> SAGNDSLPFENIQGDILVGMKKDKEKFVFFHINNATAFKSVLKTYAPANITSVATIIGPVANQPLAFVNLAFSHAGFGALNVTDDLQDTAFSDGQFKDSPNLGDDTSTWEEAFKGTNVDGVFLIGSNDESITAQYRDDLNAKFGDAWTIVYDLDSAARPGNEKGHEHFGYLDGISNPTIPGFGTPHPGQAVVDPGIIFTGRSKDPVMNRPSWALDGSFLVFRKLKQLVPEFNKYVLDNALQNQAGNLTVEEGAELLGSRMFGRWKSGAPIDLSPDFDDPALGNDIERNNNFNYSHPGSDLATDQTRCPFTAHIRKTN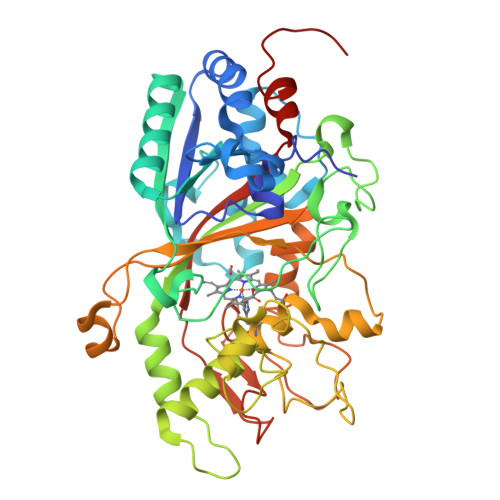PRDLEGQGLFGDTFHAIRAGTPYGPEVTDYEASSNTTTIDRGLAFVEYQSVIGNGFRFQQQAWANNPRFPFSKGPSIQLGLDPVIGQGSPRETFGLDPRNASESFTVPQVIISNGGEYFFSPSITAIVEKFAALEHHHHHH5,10-Methenyltetrahydrofolate | C20 H22 N7 O6 | 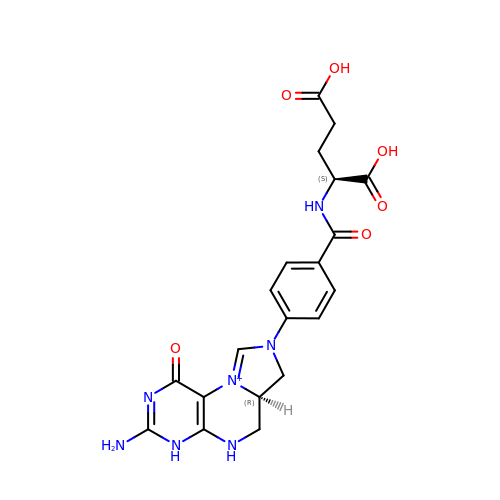MEANFMOQMXYMCT-OLZOCXBDSA-O5-phenyl-1H-indazol-3-amine | C13 H11 N3 | 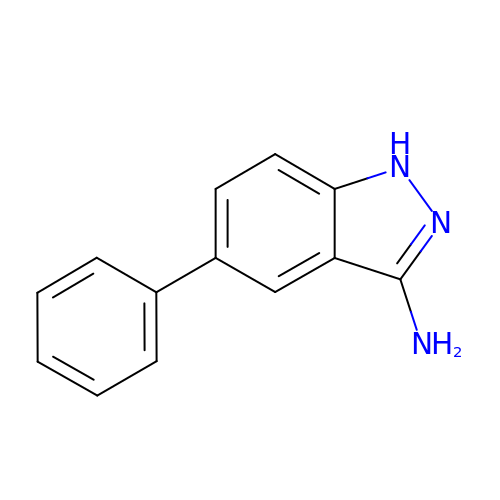ZCUSNQPYUNLATP-UHFFFAOYSA-N>MLRIIDTETCGLQGGIVEIASVDVIDGKIVNPMSHLVRPDRPISPQAMAIHRITEAMVADKPWIEDVIPHYYGSEWYVAHNASFDRRVLPEMPGEWICTMKLARRLWPGIKYSNMALYKTRKLNVQTPPGLHHHRALYDCYITAALLIDIMNTSGWTAEQMADITGRLEHHHHHH[2x]

ExoX is one of several redundant exonucleases involved in the mismatch repair system, UV repair, homologous recombination and the stabilization of tandem repeats in E. coli. Like TREX1/2, ExoX contains only an exonuclease domain; however, it can act on both ssDNA and dsDNA in a distributive manner and digests only one or two nucleotides per reaction cycle. To elucidate the mechanism by which dsDNA is recognized and processed by single-domain DnaQ members, such as ExoX and TREX1/2, we determined the structures of ExoX in complex with three distinct dsDNA substrates: 3′ overhanging duplex DNA, a 12 bp blunt-ended dsDNA and 5′ overhanging partially mismatched duplex DNA, referred to here as complexes I, II and III, respectively. The crystal structures obtained revealed that ExoX interacts with dsDNA via two DNA-binding sites, one for the substrate strand and another for the complementary strand.

In each asymmetrical unit, two protein molecules (A and B) bind to the ends of a single dsDNA molecule, thus forming a dumbbell-like structure. In complex I, the 3′ overhang is bent at an angle of 70 degrees between the first two nucleotides and extends into the active site. Outside the active site, a substrate DNA strand-binding site, mainly composed of Lys111, Tyr112 and Asn114 in the α5–α6 loop, interacts with the sugar–phosphate backbone of the substrate strand. Moreover, Lys101 and Arg104 of α5 form a specific positively charged binding site for the complementary strand. Most of the residues formed electrostatic interactions or hydrogen bonds with the DNA sugar–phosphate backbone, while few displayed electrostatic interactions or hydrogen bonding with DNA bases, which is indicative of a non–sequence-specific DNA-binding site. Strong density peaks were observed at the two conserved metal-binding sites of the DnaQ family, A and B. The intact substrate observed in our structure suggest that the metals involved are unlikely to be active metals (such as Mn2+ or Mg2+), and are probably inactive metals (such as Ni2+ or Na+). The ion bound at site A (MeA) is penta-coordinated by the side-chain oxygen atoms of Asp6, Glu8 and Asp139, one solvent water molecule and an oxygen atom of the substrate phosphate group, while the ion bound at site B (MeB) is hexa-coordinated by the side-chain oxygen atom of Asp6, three solvent water molecules and two oxygen atoms of the substrate phosphate group. The coordination of the two metal ions in ExoX is similar to that of the other members of the DEDDh subfamily, suggesting a classical phosphodiester bond cleavage mechanism for ExoX.2-amino-1,3-benzothiazol-6-ol | C7 H6 N2 O S | 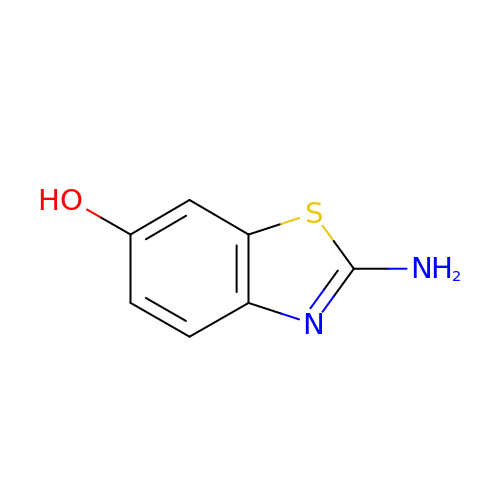VLNVTNUTGNBNBY-UHFFFAOYSA-N>MKITSSNFATIATSENFAKLSVLPKNHREPIKGLFKSAVEQFSSARDFFKNENYSKELAEKFNKEAVNEA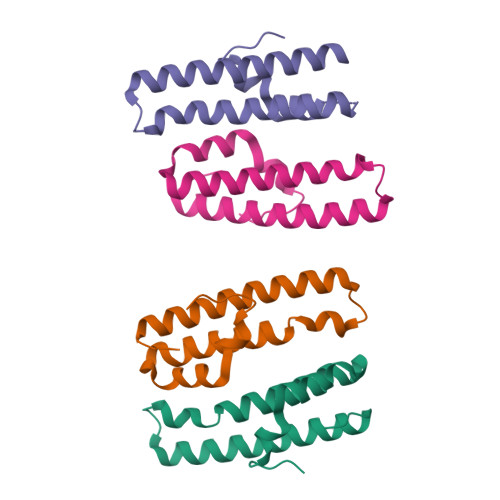VEKLQKAIDLAEKQGIQF[4x]Mycobacterium tuberculosis encodes six known TA systems with toxins belonging to the RelE-family of ribosome-dependent ribonucleases with conserved RNase T1-like folds. The RelE3(YoeB) toxin, which is mildly toxic when compared with HigB1, RelE1, or RelE2 was also shown to act as an RNase. Both RelE1 and RelE2 are acutely toxic, very similar in sequence (∼54% identity) and were proposed to have redundant functions in M. tuberculosis. In contrast, in vitro and in vivo analyses using Mycobacterium smegmatis and M. tuberculosis revealed that RelE1 is a site-specific RNase, able to cleave 16S rRNA from free 30S and formed 70S ribosomes, to release the anti-Shine–Dalgarno region and prevent translation. We show that in sharp contrast with established RelE toxins, the RelE1 RNase toxin of M. tuberculosis does not cleave mRNA during translation but instead specifically targets the small ribosomal subunit, cleaving the exposed 3′ end region of the 16S rRNA between C1517 and A1518, just upstream of the anti-SD region.

Furthermore, we solved the crystal structure of the RelE1–RelB1 complex at 2.20 Å resolution and showed that it forms a heterotetrameric complex in which the RelB1 antitoxin likely displaces the C-terminal α-helix of the partner RelE1 toxin, and identified key residues of the catalytic region that are essential for its activity. The asymmetric unit contained a heterotetrameric RelB12RelE12 protein complex. RelB12RelE12 forms a triangular (or inverted V-shaped) complex with the RelE1 toxin molecules positioned away from each other. Each RelE1 protomer, RelE1 and RelE1′, forms the expected RNase T1-like fold, and the C-terminal region of neither toxin was resolved in the structure. The RelB1 antitoxins dimerize through respective domains comprised of an N-terminal three-stranded β-sheet and the α1 helix, which then extends and wraps around cognate RelE1 toxins using helices α2, α3, and α4. Interface analysis using PISA identified salt bridges between RelE1 R50 and RelB1 D44, and RelE1 R65 and RelB1 E50, alongside RelE1 hydrophobic patches corresponding to hydrophobic faces of RelB1 α2, α3 and α4 helices, generating complementary interacting surfaces. The N-terminal dimerization domain and α2 helix of RelB1 are highly conserved, whilst α3 and α4 amino acids are not conserved. The RelE1 surface residues juxtaposed with RelB1 helix α2 are also highly conserved, but not those surface residues binding RelB1 helices α3 and α4. Helix α3 of the free RelE toxin therefore appears to be displaced by helix α3 of the cognate RelB antitoxin when forming the complex, such that antitoxicity likely operates both through sequestration and deactivation of the toxin by conformational changes. While R50A, S58A, R61A had no, or little impact, the R60A, R65A, R85A, and Y89A substitutions significantly affected RelE1 toxicity, thus highlighting R60, R65, R85, and Y89 as key catalytic residues of RelE1.

>[2x]MSDDHPYHVAITATAARDLQRLPEKIAAACVEFVFGPLLNNPHRLGKPLRNDLEGLHSARRGDYRVVYAIDDGHHRVEIIHIARRSASYRMNPCRPR;>MAVVPLGEVRNRLSEYVAEVELTHERITITRHGHPAAVLISADDLASIEETLEVLRTPGASEAIREGLADVAAGRFVSNDEIRNRYTAR[2x]>MLELLPTAVEGVSQAQITGRPEWIWLALGTALMGLGTLYFLVKGMGVSDPDAKKFYAITTLVPAIAFTMYLSMLLGYGLTMVPFGGEQNPIYWARYADWLFTTPLLLLDLALLVDADQGTILALVGADGIMIGTGLVGALTKVYSYRFVWWAISTAAMLYILYVLFFGFTSKAESMRPEVASTFKVLRNVTVVLWSAYPVVWLIGSEGAGIVPLNIETLLFMVLDVSAKVGFGLILLRSRAIFGEAEAPEPSA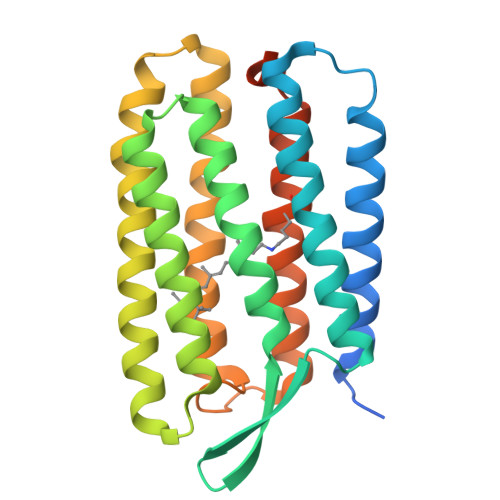GDGAAATSD[2x]> MSALYFQNLPSRPANKENYTRLLLKHINPNNKYAINPSLPLPHNKLQISSQPLMLLDDQMGLLEVSISRSSKMTNQAFLTFVTQEEADRFLEKYTTTALKVQGRKVRMGKARTNSLLGLSIEMQKKKGNDETYNLDIKKVLKARKLKRKLRSDDICAKKFRLKRQIRRLKHKLRSRKVEEAEIDRIVKEFETRRLENMKSQQ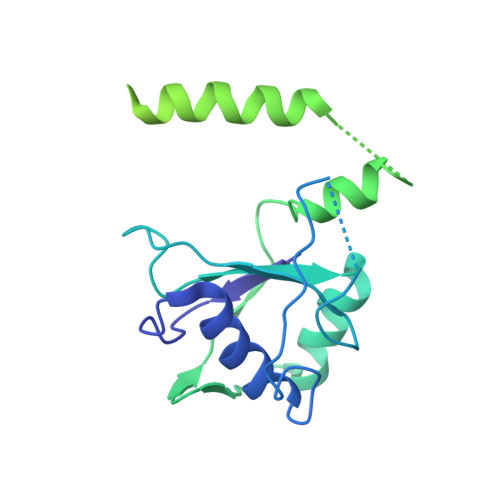ENLKQSQKPLKRAKVSNTMENPPNKVLLIQNLPSGTTEQLLSQILGNEALVEIRLVSVRNLAFVEYETVADATKIKNQLGSTYKLQNNDVTIGFAK>MSLKIAKVEALSVAMGDGTGWMPTSAFVRITAEDGTVGWGEASPMLGGIASLGVVARDIAPFLEGQEVLDHAVLLDRMMH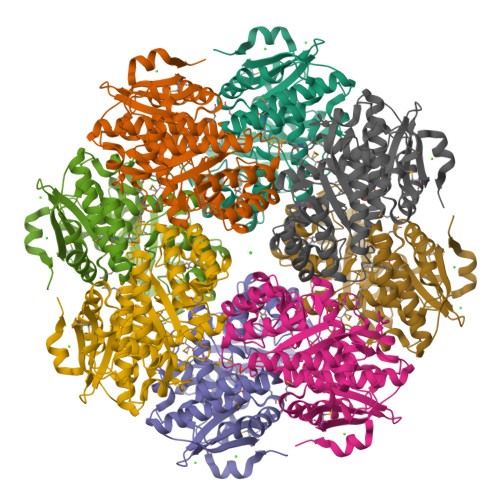RLVKLGPEGIATAALAACDIALWDLKGKLLGQPIYKLLGGAWRTRLPCYSSIGGNAARSVDEVVREVARRVEAEQPAAVKIRWDGDRTRCDVDIPGDIAKARAVRELLGPDAVIGFDANNGYSVGGAIRVGRALEDLGYSWFEEPVQHYHVGAMGEVAQRLDITVSAGEQTYTLQALKDLILSGVRMVQPDIVKMGGITGMMQCAALAHAHGVEFVPHQTQPGVGHFANIHVLSTLMHMTKPVELADRWDRGRPVFRNPAEPVDGHFALGDAPGLGIVVDEDELASRATEITVGRDQRPPAGGQYEGHHHHHH[2x]> MKQALRVAFGFLILWASVLHAEVRIVIDSGVDSGRPIGVVPFQWAGPGAAP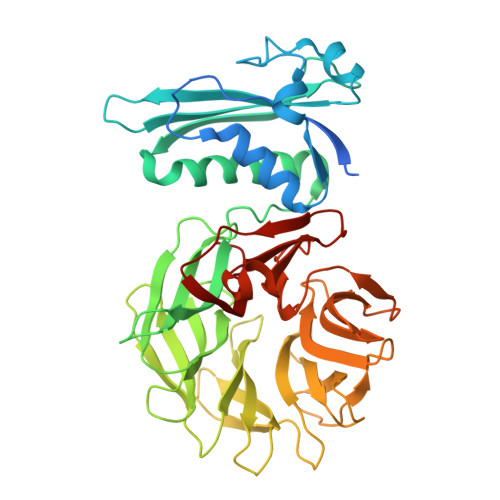EDIGGIVAADLRNSGKFNPLDRARLPQQPGSAQEVQPAAWSALGIDAVVVGQVTPNPDGSYNVAYQLVDTGGAPGTVLAQNSYKVNKQWLRYAGHTASDEVFEKLTGIKGAFRTRIAYVVQTNGGQFPYELRVSDYDGYNQFVVHRSPQCLMSPAWSPDGSKLAYVTFESGRSALVIQTLANGAVRQVASFPRHNGAPAFSPDGSKLAFALSKTGSLNLYVMDLASGQIRQVTDGRSNNTEPTWFPDSQNLAFTSDQAGRPQVYKVNINGGAPQRITWEGSQNQDADVSSDGKFMVMVSSNGGQQHIAKQDLATGGVQVLSSTFLDETPSLAPNGTMVIYSSSQGMGSVLNLVSTDGRFKARLPATDGQVKFPAWSPYL>[2x]MGSSHHHHHHSSGRENLYFQGHGTAGGGKTKISFYSYFKDNQIGEVVKGFEKKNPDITLDVQYGQDPAQYISTLQTRLAGGKPPTIFNLTMDNRTDVMKSGAALDISGEDFLDGIDDTNFALFQQDGKTYGMPVSAWVGAFFYNKDILKKAGYDKFPKTWDEFIEMGKKINSNGSTAFLEDF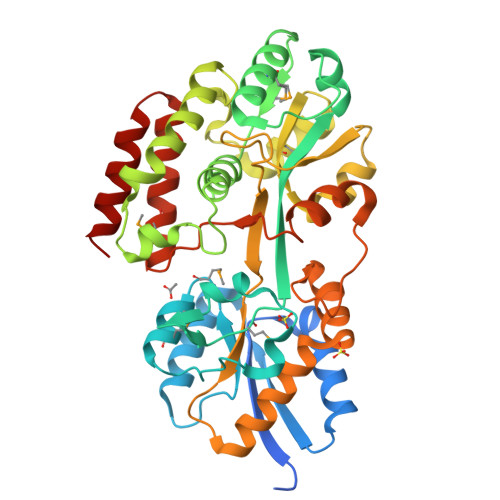NTQIAGSFTGLLASYYGEQGKSGDLDADIWSGKSTFTKDWTPVFKRWEAAAKAGVIPQKSVGLSADQVKQEFVSGNLGVMRSGPWDLPDLQKSDIDFGVAPFPAYSKEDGQWINGGPDQGFAIASRASDKEKAAAKKFLAYLNSEEGLEAFTSAAGTLSLSSKYNAEPPAELKDVVDNYFKQNKFYWVNWPKSPTVMSTEGIAQQQKIVQGQISAKDAAKALDAKWATLKGS>RLCLRNYPDTTWIGDSRSDQSRVNPQS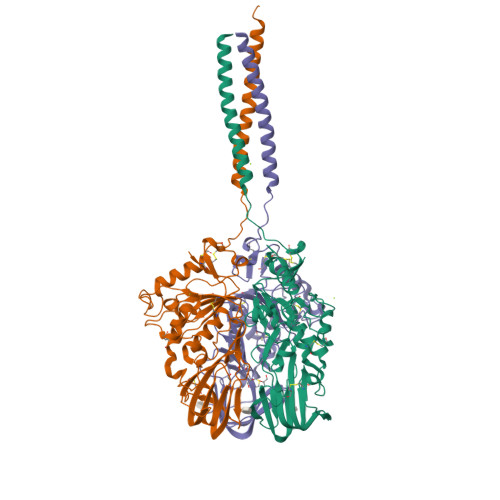LDLVTEFKGVLQAKNGNGLLKQMSGRFPSDWYTPTTKYRILYLGTNDCTDGPTDMIIPTSMTLDNAARELYLGACRGDVRVTPTFVGAAIVGLVGRTDAVTGFSVKVLTFSSPTIVVVGLNGMSGIYKVCIAATSGNVGGVKLINGCGYFNTPLRFDNFQGQIYVSDTFEVRGTKNKCVLLRSSSDTPLCSHIMRNVELDEYVDTPNTGGVYPSDGFDSLHGSASVRTFLTDALTCPDIDWSRIDAASCEYDSCPKMVKDFDQTSLGNTDTLIMREVALHKEMISKLQRDITDVKIRVDAIPPQLNQTMGRLVPR[6x]> MKAKRVQAKIEIEFPSEDVAKVVYEAVLYEHLSVPYRRSEIDFKLEGKKIILDIKATDSSALRGTVNSYLRWIKAAIDVIEVGSGSGSGSGSGMKAKRVQAKIEIEFPSEDVAKVVYEAVLYEHLS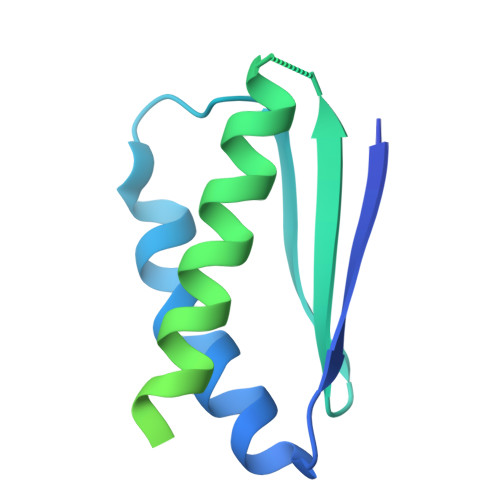VPYRRSEIDFKLEGKKIILDIKATDSSALRGTVNSYLRWIKYAIDRIEV> MGSSHHHHHHSSGNNFNNEIKLILQQYLEKFEAHYERVLQDDQYIEALETLMDDYSEFILNPIYEQQFNAWRDVEEKAQLIK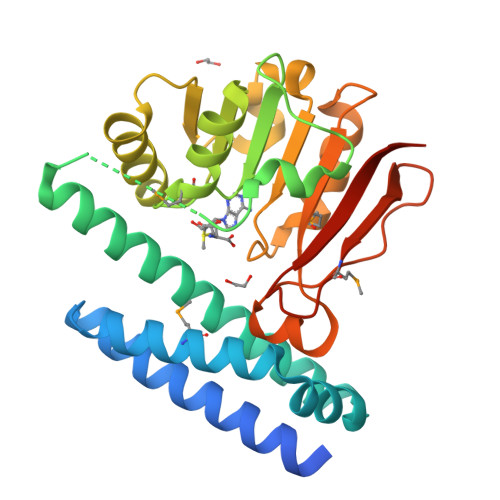SLQYITAQCVKQVEVIRARRLLDGQASTTGYFDNIEHCIDEEFGQCSITSNDKLLLVGSGAYPMTLIQVAKETGASVIGIDIDPQAVDLGRRIVNVLAPNEDITITDQKVSELKDIKDVTHIIFSSTIPLKYSILEELYDLTNENVVVAMRFGDGIKAIFNYPSQETAEDKWQCVNKHMRPQQIFDIALYKKAAIKVGITD>MRGSHHHHHHGSASEIHMTGPMCLIENTNGRLMANPEALKILSAITQPMVVVAIVGLYRTGKSYLMNKLAGKKKGFSLGSTVQSHTKGIWMWCVPHPKKPGHILVLLDTEGLGDVEKGDNQNDSWIFALAVLLSSTFVYNSIGTINQQAMDQLYYVTELTHRIRSKSSPDENENEVEDSADFVSFFPDFVWTLRDFSLDLEADGQPLTPDEYLTYSLKLKKGTSQKDETFNLPRLCIRKFFPKKKCFVFDRPVHRRKLAQLEKLQDEELDPEFVQQVADFCSYIFSNSKTKTLSGGIQVNGPRLESLVLTYVNAISSGDLPCMENAVLALAQIENSAAVQKAIAHYEQQMGQKVQLPTESLQELLDLHRDSEREAIEVFIRSSFKDVDHLFQKELAAQLEKKRDDFCKQNQEASSDRCSGLLQVIFSPLEEEVKAGIYSKPGGYRLFVQKLQDLKKKYYEEPRKGIQAEEILQTYLKSKESMTDAILQTDQTLTEKEKEIEVERVKAESAQASAKMLQEMQRKNEQMMEQKERSYQEHLKQLTEKMENDRVQLLKEQERTLALKLQEQEQLLKEGFQKESRIMKNEIQDLQTKMRRRKACTIS[6x]

Guanylate-binding proteins (GBPs) are interferon-inducible, dynamin-related GTPases that mediate cell-autonomous immunity against a wide range of microbial pathogens. Host defense against intracellular bacterial pathogens such as Shigella and Salmonella is orchestrated by human GBP1 (GBP1), a cytosolic lipopolysaccharide (LPS) immune sensor and surfactant. Upon GTP binding and hydrolysis, auto-inhibited GBP1 monomers dimerize and assemble into soluble and membrane-bound oligomers, which are crucial for innate immune responses.

Here, by applying cryo-electron tomography (cryo-ET) and subtomogram averaging (StA) on GBP1-coated liposomes and single particle analysis (SPA) on self-polymerized GBP1, we report an outstretched, dimeric conformation of GBP1 oligomerized on a lipid surface and in its polymeric state in solution. The GDP•AlFx-bound GBP1 coatomer was well recognizable in cryo-ET volumes of BPL liposomes. The protein coat had an average height of 28.3 nm ± 1.6 nm, which agrees well with the theoretical dimension of a dimeric, outstretched GBP1 dimer (~28.8 nm). We further performed subtomogram averaging which resulted in a map of membrane-bound GBP1 dimers at a moderate resolution of ~26 Å (Figs. 1F and EV1, Movie EV1). Although the map did not allow for a detailed molecular fitting of the GBP1 dimer, it suggested the potential oligomerization interfaces: the MD and GED were apparently not involved in higher order assembly, based on the absence of density between these elements outside the dimer. In contrast, the dimeric LG domains displayed lateral contacts mediating the formation of a two-dimensional protein lattice. Within the coatomer, the overall shapes of the LG domain and MD match well with the recently published crystal structure of the GBP5 dimer and the cryo-EM structure of the GBP1 dimer, suggesting that the coatomer is comprised of dimeric building blocks with crisscrossed MDs that are extended by elongated GEDs. The GEDs extend in parallel toward the membrane surface, allowing the C-terminal farnesyl moiety to insert into the lipid bilayer. We show that the peripheral helix α4’ in the LG domain is critical for establishing the oligomeric interface and facilitates the formation of an antimicrobial protein coat. The farnesyl moiety can insert into the membrane, while helix α4’ is available to form a stable oligomeric interface via the LG domains.>[4x]ELQARSRIKWAIDYITKYFFTEGIYLQKRQR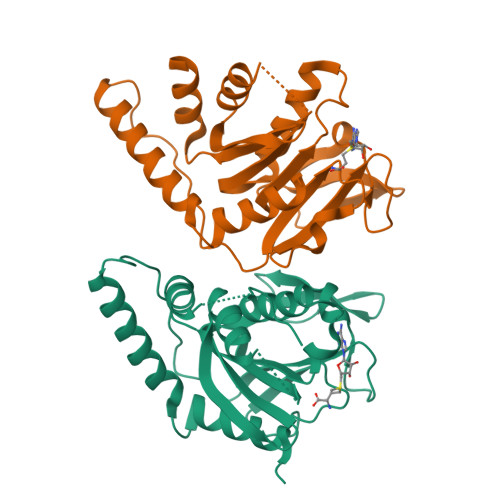EQRLLESYRAEGKLGEVQCRLMEEPPDRLHVLDVGSCFNPFSSAPHLEVTALDLCPATEDVLQADFLKVEVVPGIREPELEEGSVRRLPASHYECVIFSLLLEYMPSAEQRLQCCLQAYDLLLPEGILVLITPDSQHVGKNAHLMKNWRYSLARIGLLRVRFEKLPHISCMVFRKAISRELSQHWASIHREEGMCEEIRIPQDDS O2-tert-butyl O3-ethyl 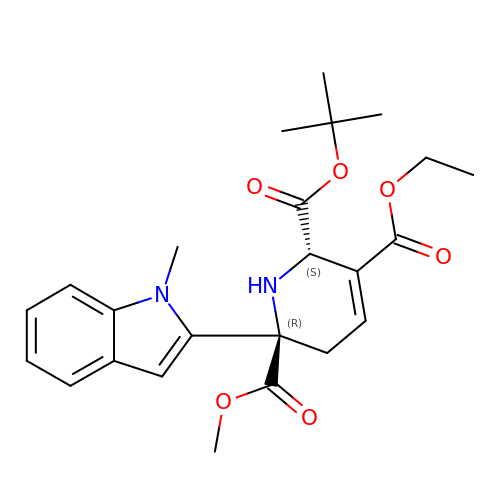O6-methyl (2S,6R)-6-(1-methylindol-2-yl)-2,5-dihydro-1H-pyridine-2,3,6-tricarboxylate | C24 H30 N2 O6 | KITXNGADRUMEPM-YADARESESA-N> MTVTRRHFLKLSAGAAVAGAFTGLGLSLAPTVARAELQKLQWAKQTTSICCYCAVGCGLIVHTAKDGQGRAVNVE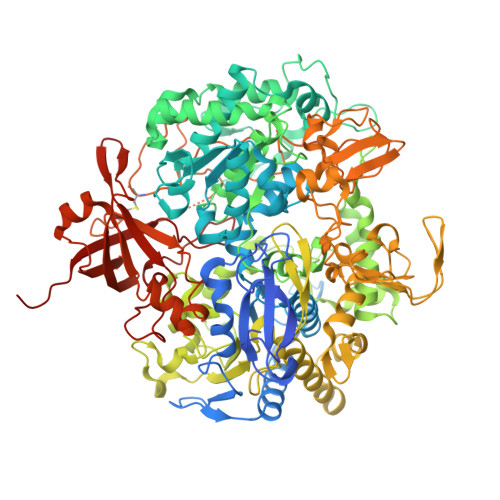GDPDHPINEGSLCPKGASIFQLGENDQRGTQPLYRAPFSDTWKPVTWDFALTEIAKRIKKTRDASFTEKNAAGDLVNRTEAIASFGSAAMDNEECWAYGNILRSLGLVYIEHQARIUHSPTVPALAESFGRGAMTNHWNDLANSDCILIMGSNAAENHPIAFKWVLRAKDKGATLIHVDPRFTRTSARCDVYAPIRSGADIPFLGGLIKYILDNKLYFTDYVREYTNASLIVGEKFSFKDGLFSGYDAANKKYDKSMWAFELDANGVPKRDPALKHPRCVINLLKKHYERYNLDKVAAITGTSKEQLQQVYKAYAATGKPDKAGTIMYAMGWTQHSVGVQNIRAMAMIQLLLGNIGVAGGGVNALRGESNVQGSTDQGLLAHIWPGYNPVPNSKAATLELYNAATPQSKDPMSVNWWQNRPKYVASYLKALYPDEEPAAAYDYLPRIDAGRKLTDYFWLNIFEKMDKGEFKGLFAWGMNPACGGANANKNRKAMGKLEWLVNVNLFENETSSFWKGPGMNPAEIGTEVFFLPCCVSIEKEGSVANSGRWMQWRYRGPKPYAETKPDGDIMLDMFKKVRELYAKEGGAYPAPIAKLNIADWEEHNEFSPTKVAKLMNGYFLKDTEVGGKQFKKGQQVPSFAFLTADGSTCSGNWLHAGSFTDAGNLMARRDKTQTPEQARIGLFPNWSFCWPVNRRILYNRASVDKTGKPWNPAKAVIEWKDGKWVGDVVDGGGDPGTKHPFIMQTHGFGALYGPGREEGPFPEHYEPLECPVSKNPFSKQLHNPVAFQIEGEKKAVCDPRYPFIGTTYRVTEHWQTGLMTRRCAWLVEAEPQIFCEISKELAKLRGIGNGDTVKVSSLRGALEAVAIVTERIRPFKIEGVDVHMVGLPWHYGWMVPKNGGDTANLLTPSAGDPNTGIPETKAFMVDVRKVWSHP>[2x]SMIPHSWICEKHILWLKDYKNSSNWKLFKECWKQGQPAVVSGVHKKMNISLWKAESISLDFGDHQADLLNCKDSIISNANVKEFWDGFEEVSKRQKNKSGETVVLKLKDWPSGEDFKTMMPARYEDLLKSLPLPEYCNPEGKFNLASHLPGFFVRPDLGPRLCSAYGVVAAKDHDIGTTNLHIEVSDVVNILVYV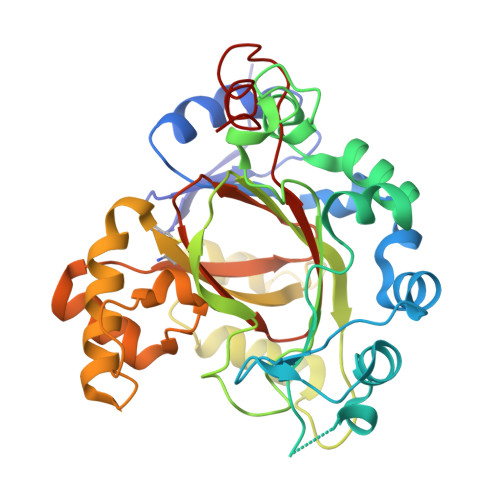GIAKGNGILSKAGILKKFEEEDLDDILRKRLKDSSEIPGALWHIYAGKDVDKIREFLQKISKEQGLEVLPEHDPIRDQSWYVNKKLRQRLYEEYHVRTCTLIQFLGDAIVLPAGALHQVQNFHSCIQVTEDFVSPEHLVESFHLTQELRLLKE>MNIEKTRFCINRKIAPGLSIEAFFRLVKRLEFNKVELRNDMPSGSVTDDLNYNQVRNLAEKYGLEIVTINAVYPFNQLTEEVVKKTEGLLRDAQGVGARALVLCPLNDGTIVPPEVTVEAIKRLSDLFARYDIQGLVEPLGFRVSSLRSAVWAQQLIREAGSPFKVLLDTFHHHLYEEAEKEFASRIDISAIGLVHLSGVEDTRPT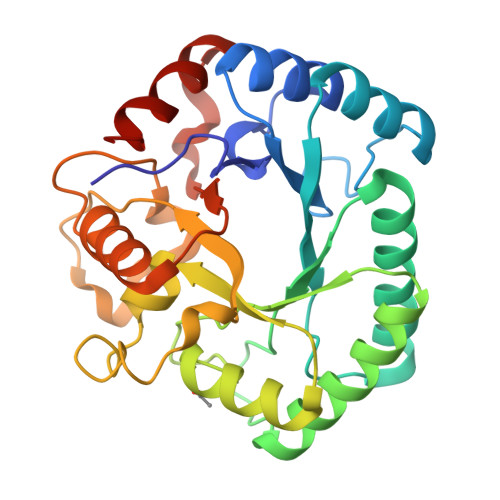EALADEQRIMLSEKDVMQNYQQVQRLENMGYRGIYAFEPFSSQLASWSEAEIEEQINRSVSLLLQ[2x]>GASDFQTGIHKIVIQQSGDTDSFEVSVSIGGADKGGPAKLYNDKGEYIGDSYSAQIRTATMSCCTNGNAF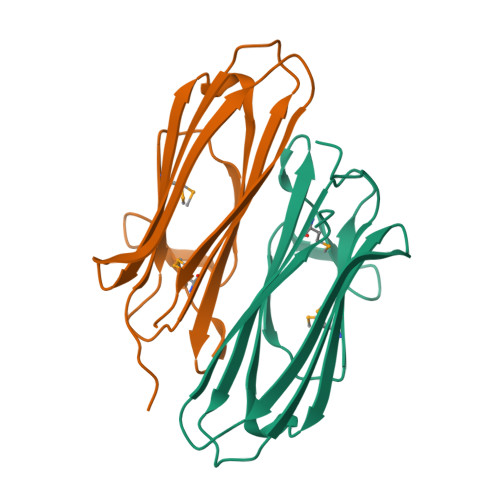FMTCAGSVSSISEAGKRLHITVIGYIDDKEVNRLEKEYITDGNTLIETFSVSTKEI[2x]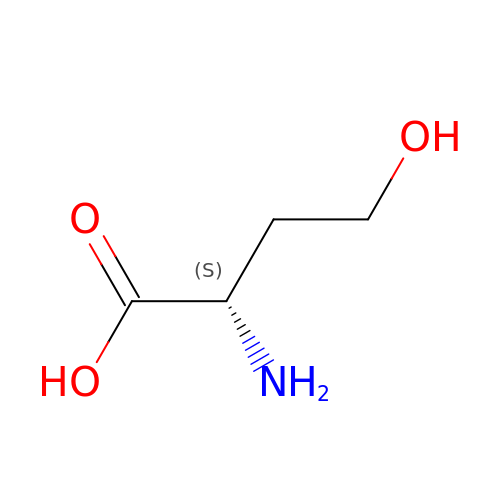L-HOMOSERINE | C4 H9 N O3 | UKAUYVFTDYCKQA-VKHMYHEASA-N>HSSGLVPRGSHMSQERILDGEEDEINHKIFDLKRTLKDNLPLDRDFIDRLKRYFKDPSDQVLALRELLNEKDLTAEQVELLTKIINEIISGSEKSVNAGINSAIQAKLFGNKMKLEPQLLRACYRGFIMGNISTTDQYIEWLGNFGFNHRHTIVNFVEQSLIVDMDSEKPSCNAYEFGFVLSKLIAIKMIRTSDVIFMKKLESSSLLKDGSLSAEQLLLTLLYIFQYPSESEQILTSVIEVSRASHEDSVVYQTYLSSVNESPHDIFKSESEREIAINILRELVTSAYKKELSR[2x]

The pathogenicity of Shigella sp. is dependent on a complex macromolecular machine, the type 3 secretion system (T3SS), that delivers into host cells a set of effector proteins required for invasion. Blockage of effector secretion before host cell contact is mediated, in part, by a protein that has been proposed to act as either a physical impediment to the entrance to the secretion apparatus, or as a gatekeeper that determines substrate hierarchy. Across bacterial species, this protein (known as MxiC in Shigella sp.) possesses only weak sequence homology and in some species exists as two separate polypeptide chains (e.g., in Yersinia sp. the homologue consists of YopN and TyeA). MxiC is an elongated rod-shaped molecule with a long axis of 86 Å.

In order to improve the quality of MxiC crystals, a shortened construct encompassing residues 74–355 (MxiCNΔ73) was expressed, purified and subjected to crystallization trials. Reductive methylation of MxiCNΔ73 yielded crystals that diffracted to higher resolution: 2.85 Å and 2.5 Å in space groups P212121 and P222, respectively. The first and last domains consist only of the X-bundle motif while the central domain also possesses a bent helix (α5) that is packed against domain 1. It is the first two domains of MxiC that are equivalent to YopN while the third domain of MxiC, equivalent to TyeA, is connected to domain 2 via a ten-residue linker. There are a total of seven independent MxiC molecules in the crystallographic asymmetric units of the three refined crystal forms. These structures reveal that, although the fold of each domain is maintained in all structures (rmsd over Cα atoms of domains 1, 2 and 3 are 0.5 Å, 0.9 Å and 0.8 Å, respectively), there is some flexibility at the interfaces between domains resulting in a “wobble” of the terminal domains about the central domain (rmsd over all Cα atoms of 1.4 Å). Interestingly, mapping of sequence conservation onto the structure across the more closely related Salmonella, Burkholderia and Shigella species reveals a hydrophobic patch on the surface of the central domain consisting of residues Leu222, Met226, Gly239, Leu242 and Leu245 (red circle). This region is buried by crystal contacts in all seven independent molecules of MxiC in the P212121, P222 and P43212 crystal forms, suggesting that this region may be a “hot spot” for protein–protein interactions. Surprisingly, the most striking difference instead involves the long á-helix (α9) in the central domain of MxiC, which is straight in all of our MxiC structures, but possesses a sharp kink in YopN when complexed with TyeA. It is the straightening of this helix that results in a reorientation of the C-terminal domain of MxiC, compared with TyeA, and opens one face of the molecule.> HMASMKKKGSVVIVGRINLSGDTAYAQQTRGEEGCQETSQTGRDKNQVEGEVQIVSTATQTFLATSINGVLWTVYHGAGTRTIASPKGPVTQMYTNVDKDLVGWQAPQGSRSLTPCTCGSSDLYLVTRHADVIPVRRRGDSRGSLLSPRPISYLKGSSGGPLLCPAGHAVGIFRAAVSTRGVAKAVAFIPVESLETTMRS

The NS3/4A protease is an excellent target for developing DAAs against HCV, and protease inhibitors have been a key component of most combination therapies. This essential protease cleaves the HCV polyprotein into functional units necessary for viral replication and maturation. Structurally Asp168 is a critical residue that contributes to an active-site electrostatic network necessary for efficient inhibitor binding. We rationally designed HCV protease inhibitors that retain potency while fitting within the substrate envelope to avoid resistance, particularly against D168A, which confers high-level resistance to current HCV PIs.

To overcome the vulnerability caused by the P2–P4 macrocycle of grazoprevir, we replaced it with a P1–P3 macrocycle previously used in danoprevir to design inhibitors that can avoid resistance while retaining potency. The resulting inhibitor, 5172-mcP1P3, was less susceptible to single-site RASs, particularly A156T, and the crystal structures validated that the binding mode of the P2 quinoxaline moiety stacking against catalytic residues was retained. Further optimization by modifications at the 3-position of the P2 quinoxaline moiety to decrease interactions with the S2 subsite residues Arg155 and Ala 156 revealed that compounds with a smaller methyl group at this position retains better activity against resistant variants. The resulting inhibitor with the optimized P2 quinoxaline achieved an improved resistance profile and avoided susceptibility to RASs. Relocating the macrocyle to fit within the substrate envelope in 5172-mcP1P3 (35) and the closely related parent compound indeed achieved a flatter resistance profile than that of grazoprevir but unfortunately resulted in potency loss against the WT protease in enzymatic assays. The parent compound, which has a P1–P3 macrocycle, fits better in the substrate envelope. Starting with the parent compound, which has an optimized P2 quinoxaline, the design aimed to fill the S4 and S5 pockets under the restraints of the substrate envelope, with the goal of gaining potency and avoiding resistance. All of the P4 inhibitors were also tested against the D168A RAS and except for P4-2 performed better than the parent compound and grazoprevir (both ∼50 nM), ranging in potency from 2 to 36 nM. The reduced potency of the inhibitors against the D168A variant, as with grazoprevir, is due to the disruption of the electrostatic network involving the Arg155 side chain as a result of the D168A substitution.GLYOXYLIC ACID | C2 H2 O3 | 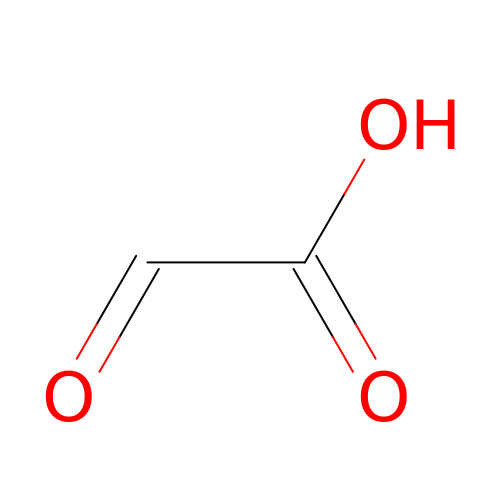HHLFWLYXYJOTON-UHFFFAOYSA-N> GPIDEEDDDLVGVSVRPKVPLRTMSYKLAIDMSHFIKEKGGLEGIYYSARRHRILDIYLEKEEGIIPDWQDYTSGPGIRYP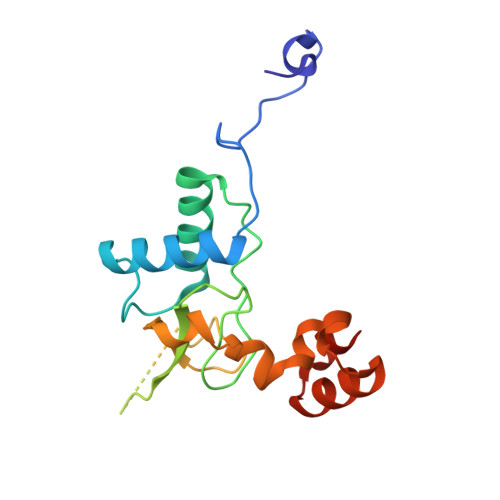KTFGWLWKLVPVNVSDEAQEDEEHYLMHPAQTSQWDDPWGEVLAWKFDPTLAYTYEAYVRYPEEFGSKSGLSEEEVRRRLTARGLLNMADKKETR>MSTGIEIQGICAPEFTKVRDAFAANFKDGKEVGASFGLAIEGEIVVDLWGGFADAGRSRPWRSDTLINTYSTTKGMAATVVGVLADEGLIDYNARVADYWPEFAAAGKKDVTVAQLLSHQAGICGPRERVEMADLYDWDKLCAMLAAQWPFFEPGTANGYHAVVFGHIAGEVARRVTGRTKSLGQLFAEKVASPIGAGNDYYIGLPASEDHRVAEMLPVIGSEQLGTGLGGKKRMSDALYCAMAHPPLTAHIANDRAWRAAEVPGANGQGNGRGIAKVYGALANGGTLGGTRIISAKGIAEMTREECFRKDEVIGVRMRWSRGFILNKAELYGPNPDAFGH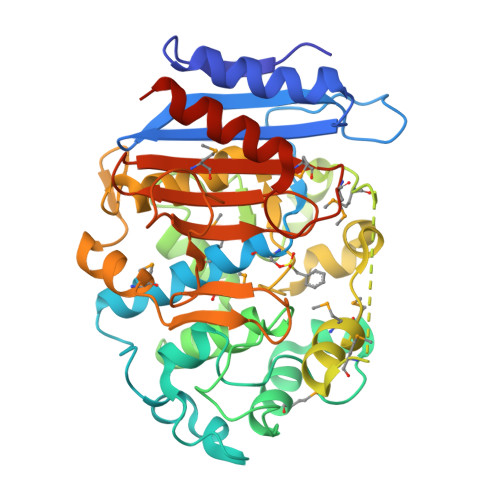SGWGGSFGFADTKARLGMGYAMNQMDTNIFGDPRGVRLIEAAYRCLPNSLEHHHHHH[2x]(6,7-DIHYDRO-5H-CYCLOPENTA[D]IMIDAZO[2,1-B]THIAZOL-2-YL]-4,7-DIHYDRO[1,4]THIAZEPINE-3,6-DICARBOXYLIC 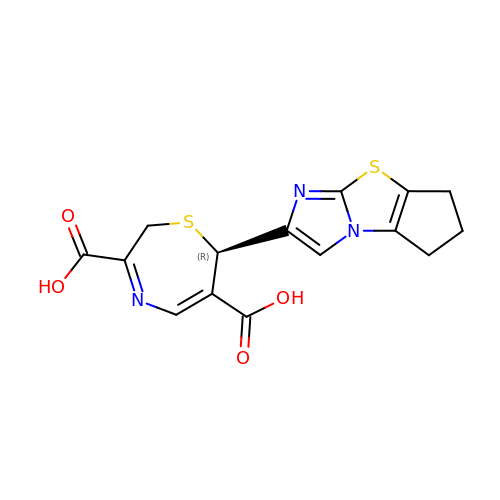ACID | C15 H13 N3 O4 S2 | CHNMLWCTGYMVFH-GFCCVEGCSA-N> SASEEQVAQDTEEVFRSYVFYRHQQEQEAEGVAAPADPEMVTLPLQP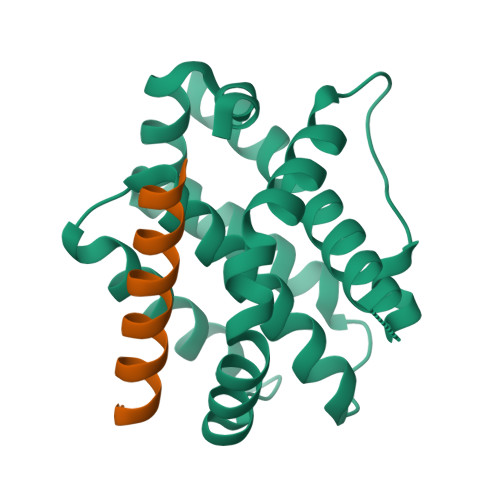SSTMGQVGRQLAIIGDDINRRYDSEFQTMLQHLQPTAENAYEYFTKIATSLFESGINWGRVVALLGFGYRLALHVYQHGLTGFLGQVTRFVVDFMLHHCIARWIAQRGGWVAALNLCNG;> EDIIRNIARHLAQWGDSMDRSW>[4x]PQFDILCKTPPKVLVRQFVERFERPSGEKIALCAAELTYLCWMITHNGTAIKRATFMSYNTIISNSLSFDIVNKSLQFKYKTQKATILEA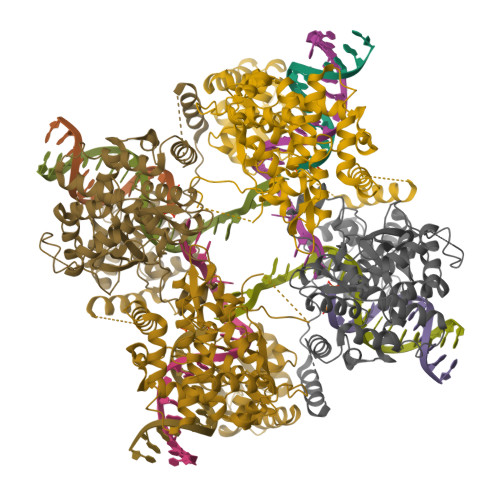SLKKLIPAWEFTIIPYYGQKHQSDITDIVSSLQLQFESSEEADKGNSHSKKMLKALLSEGESIWEITEKILNSFEYTSRFTKTKTLYQFLFLATFINCGRFSDIKNVDPKSFKLVQNKYLGVIIQCLVTETKTSVSRHIYFFSARGRIDPLVYLDEFLRNSEPVLKRVNRTGNSSSNKQEYQLLKDNLVRSYNKALKKNAPYSIFAIKNGPKSHIGRHLMTSFLSMKGLTELTNVVGNWSDKRASAVARTTYTHQITAIPDHYFALVSRYYAYDPISKEMIALKDETNPIEEWQHIEQLKGSAEGSIRYPAWNGIISQEVLDYLSSYINRRI N-[9-(2-carboxyphenyl)-6-(diethylamino)-3H-xanthen-3-ylidene]-N-ethylethanaminium | C28 H31 N2 O3 | 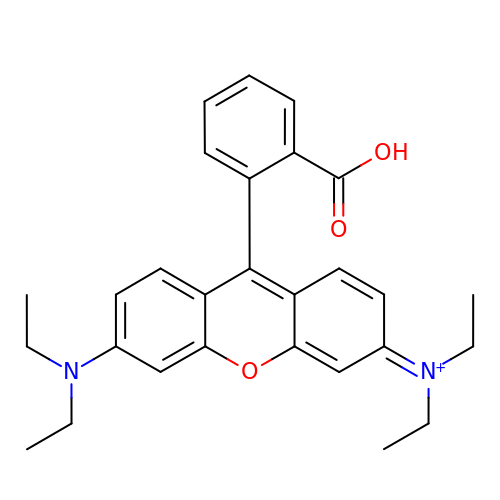CVAVMIODJQHEEH-UHFFFAOYSA-O> MSELYQAKSETRSTITSSLKGIQPYKPTKATIWSRADALKVNEYDPTTTQPLVSGDFPVMSDEVFIWDTMPLRDIDGNIASVNGWSVIFTLTADRNPTAPEYQDEQGNYDI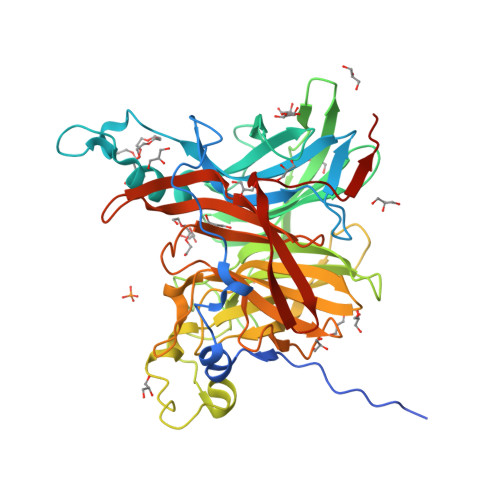TLDWNDRHGRAKMYFWYSRTGKDWIIGGRVMAEGVSPTAREWSGTPVLLNERGEIDLYYTAVTPGATVVKVRGRVVTTENGVEMVGFKKVKSLFEADGKMYQTESQNPYWAFRDPCPFRDPKSGKLYMLFEGNVAGERGSHVVGPDELGDVPPGYEDAGNSHFQTGCIGIAVCRDEDGDDWELLPPLITAVGVNDQTERPHFVFQDGKYYLFTISHKFTYGDGLTGPDGVYGFVSENLFGPYVPLNGSGLVLGNPPSQPYQTYSHYVMPNGLVTSFIDSVPTGEDSYRIGGTEAPTVLIKLKGAQTFVLEEFDYGYIPPMIDVKVEHHHHHH>GAAADLDTQRSDIATLLKTSLRKGDTWYLVDSRWFKQWKKYVGFDSWDKYQMGDQNVYPGPIDNSGLLKDGDAQSLKEHLIDELDYILLPTEGWNKLVSWYTLMEGQEPIARKVVEQGMFVKHCKVEVYLTELKLCENGNMNNVVTRRFSKADTIDTIEKEIRKIFSIPDEKETRLWNKYMSNTFEPLNKPDSTIQDAGLYQGQ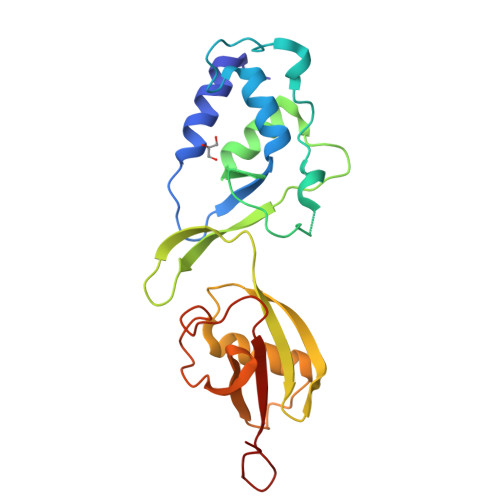VLVIEQKNEDGTWPRG[2x]> GSMLIDAIHGAKMSTKLLVSLKVLVIQLNPQIGQVDQTIKRTWSILDKVTKSATYVKPDIILFPEFALTGYSFHARKDILPYVTKKDEGPSFELAKSISEKFQCYTIIGYPEEDDEQKLYNSALVVNPQGGQIFNYRKTFLYDTEMNWDCEENPEGFQTFPMDFSKCAKLSNEDSYNRDVTLKASIGISMDLSPYKFMAPFNHFEFSSFCVDNNVELILCPMAWLNSTSITDKQTLHNNSLLEAAKNKIAFALKEQGLPLAGSQGIYQLKIGDSQRTPRVPSDDSTSEYKDMDEPDMSNVNYWILRFFPFLYFKLRINWFKNSSLIESILGKTRMPLDHEYYKDG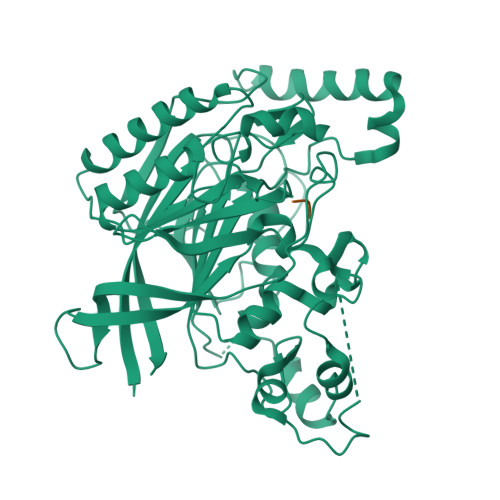KHKEDTIDLLDSEEVIKDTVLEKTFLGTSLGQPWKFQGKNAILVLANRCGTEDGTTIFAGSSGIYKFNGKKPKGSQDDDESSLDSLNESVELLGNLGKGLEGAILREVQFEVFR;> NEA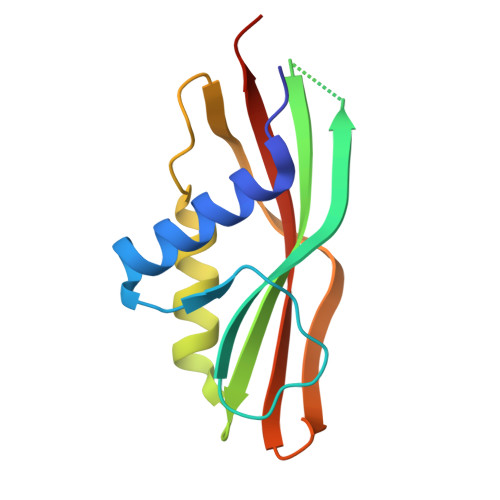> MKSLSFMRVLEAVRTMLQEKGGLDVSIVMRNQVEMPTTMIEMIDQEEEESQTAWKEKYRFAIHHYTNEQDLAGVEMIDTLIQMGFILPEGYKLVAVRHCGKQNLVKENTLIHAKTSFEVSICRELKVKI>GGFSQSCLPNWIMHGKSCYLFSFSGNSWYGSKRHCSQLGAHLLKIDNSKEFEFIESQTSSHRINAFWIGLSRNQSEGPWFWEDGSAFFPNSFQVRNAVPQESLLHNCVWIHGSEVYNQICNTSSYSICEKELKHHHHHH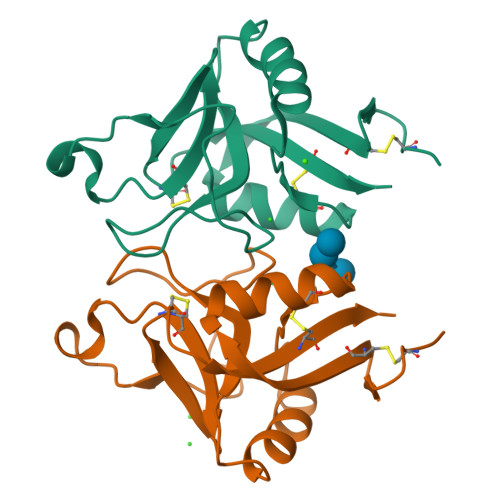[2x]N-CYCLOHEXYL-N'-DECYLUREA | C17 H34 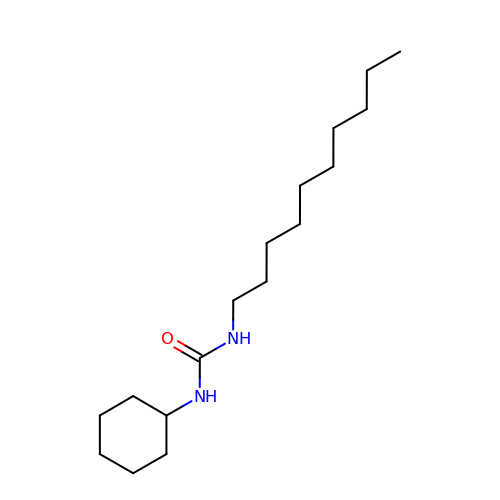N2 O | LPXYBLIRYGCMPQ-UHFFFAOYSA-N> GPRKITIALLGLDNAGKTTLLNSIQGEVDRDTTPTFGFNSTTLNEGKYKIEVFDLGGGKNIRGVWKKYLAEVHAIVYVVDAADPGRFE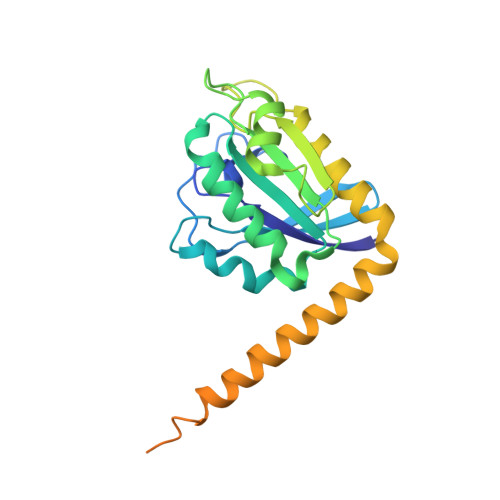ESKMTMAEVLENQFMRDKPICIFANKQDLPTAAPAAEVVKGLGLATCRNSHNVFPCTAKMPAGQDVDHRLRDGLKWLVGTVDREFGRLDPRVQTEAEEVRQEEARKKKEREERLRKQREERLRQQKEEEERAREVEKENELHDGKAPSLLAAGGGVVGAAAAGVNGVMVDEQQEL> TWLSDFPQAWAETGGMGLAVRQAPLIIPLKATSTPVSIKQYPMSQEARLGIKPHIQRLLDQGILVPCQSPWNTPLLPVKKPGTNDYR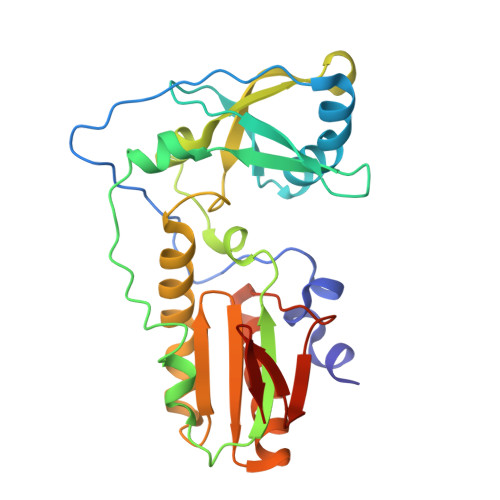PVQDLAEVNKRVEDIHPTVPNPYNLLSGLPPSHQWYTVLDLKDAFFCLRLHPTSQPLFAFEWRDPEMGISGQLTWTRLPQGFKNSPTLFDEALHRDLADFRIQHPDLILLQYVDDLLLAATSELDCQQGTRALLQTLGNLGYRASAKKAQICQKQVKYLGYLLKEGQR(5R)-2-[(2-fluorophenyl)amino]-5-(1-methylethyl)-1,3-thiazol-4(5H)-one 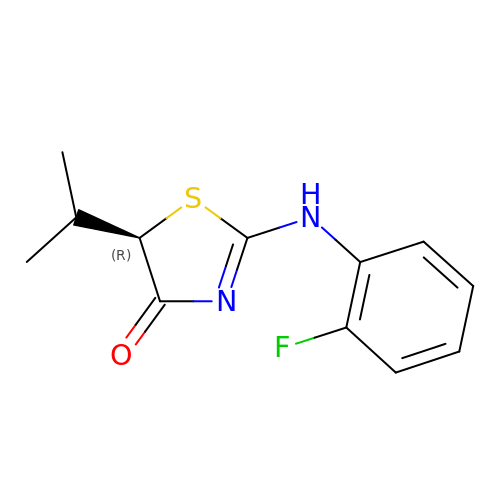| C12 H13 F N2 O S | OJJBBNIYQKFZDK-SNVBAGLBSA-N>TFDYSVDCDGAILGAAVNGKKSAHGSPTFWMGSHEVNGTWMIHTLETLDYKECEWPLTHTIGTSVEESDMFMPRSIGGPVSSHNRIPGYKVQTNGPWMQVPLEVKREVCPGTSVVVDSNCDGRGKSTRSTTDSGKIIPEWCCRSCTMPPVSFHGSD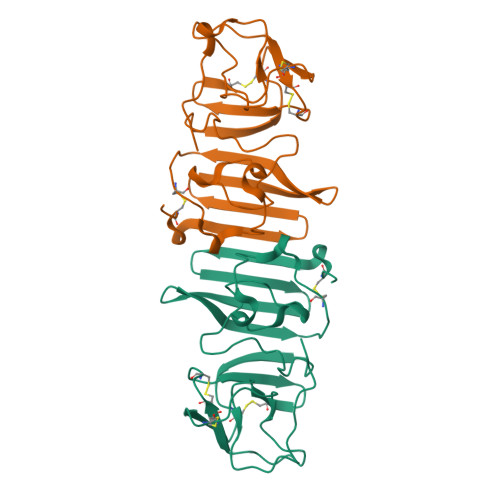GCWYPMEIRPMKTSDSHLVRSWVTA[4x]>[2x]MTTNTIMEQEARTAPQKIAEQLLANDAITESLGSVLREFKPKFVMIVGRGSSDHAGVFAKYLFEIEASIPTFAAAPSVASVYGK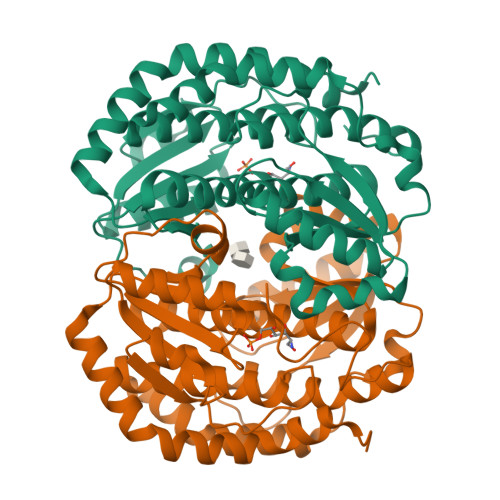TLKLAGGLVIVISQSGRSPDILAQARMAKNAGAFCVALVNDETAPIKDIVDVVIPLRAGEEKAVAATKSYLATLSALLQVAAKWTQNESLVEAVNSLPQALQAAVDAEPQLRAGSLTDVKNLVVLGRGFGYAVSKEIALKLKEVCAIHAEAFSSAEFLHGPVTLVEKKLSILDVCIRDESYGSHVEQIANVKQRGANLIHLHQTSADIHPRIAPLALLQRFYIDVAAVAIALGINPDKPAGLKKVTQTL>QEGLDFPEYDGVDRVINVNAKNYKNVFKKYEVLALLYHEPPEDDKASQRQFEMEELILELAAQVLEDKGVGFGLVDSEKDAAVAKKLGLTEVDSMYVFKGDEV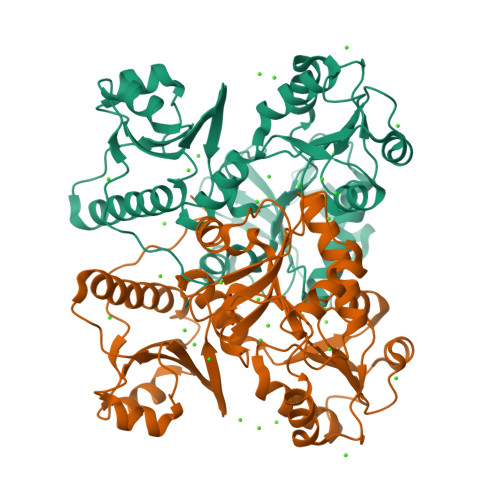IEYDGEFSADTIVEFLLDVLEDPVELIEGERELQAFENIEDEIKLIGYFKSKDSEHYKAFEDAAEEFHPYIPFFATFDSKVAKKLTLKLNEIDFYEAFMEEPVTIPGKPNSEEEIVNFVEEHRRSTLRKLKPESMYETWEDDMDGIHIVAFAEEADPDGFEFLETLKAVAQDNTENPDLSIIWIDPDDFPLLVPYWEKTFDIDLSAPQIGVVNVTDADSVWMEMDDEEDLPSAEELEDWLEDVLEGEINTEDDDDDDDD[4x]> SLSCRPPMVKLVCPADNLRAEGLECTKTCQNYDLECMSMGCVSGCLCPPGMVRHENRCVALERCPCFHQGKEYAPGETVKIGCNTCVCQDRKWNCTDHVCDATCSTIGMAHYLTFDGLKYLFPGECQYVLVQDYCGSNPGTFRILVGNKGCSHPSVKCKKRVTILVEGGEIELFDGEVNVKRPMKDETHFEVVESGRYIILLLGKALSVVWDRHLSISVVLKQTYQEKVCGLCGNFDGIQNNDLTSSNLQVEEDPVDFGNSWKVSSQCADTRKVPLDSSPATCHNNIMKQTMVDSSCRILTSDVFQDCNKLVDPEPYLDVCIYDT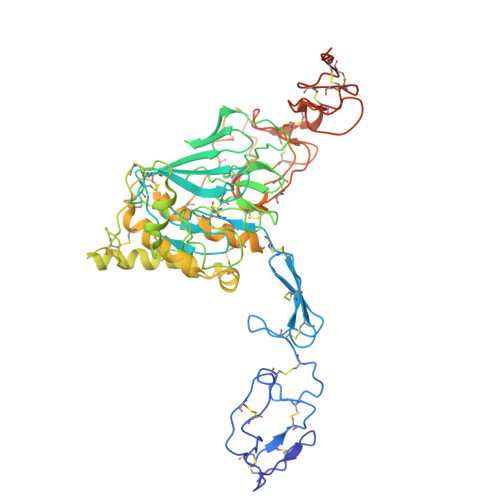CSCESIGDCACFCDTIAAYAHVCAQHGKVVTWRTATLCPQSCEERNLRENGYECEWRYNSCAPACQVTCQHPEPLACPVQCVEGCHAHCPPGKILDELLQTCVDPEDCPVCEVAGRRFASGKKVTLNPSDPEHCQICHCDVVNLTCEACQEPGGLVVPPHHHHHH>GHMDNLVLIRMKPDENGRFGFNVKGGYDQKMPVIVSRVAPGTPADLCVPRLNEGDQVVLINGRD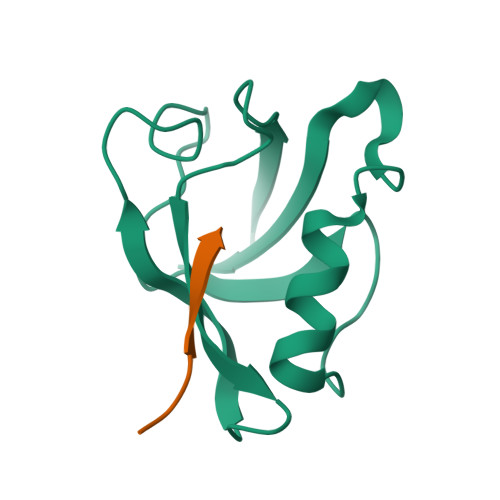IAEHTHDQVVLFIKASCERHSGELMLLVRP[4x];>[4x]TRRETQL> ANIVGGIEYSINNASLCSVGFSVTRGATKGFVTAGHCGTVNATARIGG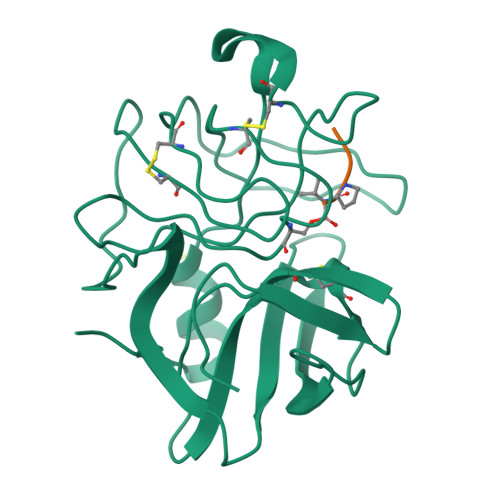AVVGTFAARVFPGNDRAWVSLTSAQTLLPRVANGSSFVTVRGSTEAAVGAAVCRSGRTTGYQCGTITAKNVTANYAEGAVRGLTQGNACMGRGDSGGSWITSAGQAQGVASGGNVQSNGNNCGIPASQRSSLFERLQPILSQYGLSLVTG;> XAAPV>MADYKDDDDKSGRMATCWQALWAYRSYLIVFFVPILLLPLPILVPSKEAYCAYAIILMALFWCTEALPLAVTALFPLILFPMMGIVDASEVAVEYLKDSNLLFFGGLLVAIAVEHWNLHKRIALRVLLIVGVRPAPLILGFMLVTAFLSMWISNTATSAMMVPIAHAVLDQLHSSQASSNVEEGSNNPTFELQEPSPQKEVTKLDNGQALPVTSASSEGRAHLSQKHLHLTQCMSLCVCYSASIGGIATLTGTAPNLVLQGQINSLFPQNGNVVNFASWFSFAFPTMVILLLLAWLWLQILFLGFNFRKNFGIGEKMQEQQQAAYCVIQTEHRLLGPMTFAEKAISILFVILVLLWFTREPGFFLGWGNLAFPNAKGESMVSDGTVAIFIGIIMFIIPSKFPGLTQDPENPGKLKAPLGLLDWKTVNQKMPWNIVLLLGGGYALAKGSERSGLSEWLGNKLTPLQSVPAPAIAIILSLLVATFTECTSNVATTTIFLPILASMAQAICLHPLYVMLPCTLATSLAFMLPVATPPNAIVFSFGDLKVLDMARAGFLLNIIGVLVIALAINSWGIPLFSLHSFPSWAQSNTTAQCLPSLANTTTPSP[2x]

The solute carrier 13 (SLC13) family comprises electrogenic sodium ion–coupled anion cotransporters, segregating into sodium ion–sulfate cotransporters (NaSs) and sodium ion–di- and–tricarboxylate cotransporters (NaDCs). NaS1 and NaDC1 regulate sulfate homeostasis and oxidative metabolism, respectively. From an overall view, both the NaDC1 and NaS1 form a homodimer, and each protomer consists of 11 TMDs. The rest TMDs form the core domain that is responsible for substrate recognition and conformational change to complete the transport cycle.

In addition, we elucidated NaDC1’s outward-facing conformation, encompassing apo, citrate-bound, and N-(p-amylcinnamoyl) anthranilic acid (ACA) inhibitor–bound states. In this section, we will predominantly focus on the detailed structural analysis of the apo structure of NaDC1. Notably, the intracellular loop (residue 165 to 212 amino acids) of NaDC1 that connects the HPin and TM5 was poorly resolved because of its flexibility. In addition, the rest sequences of NaDC1 were clearly resolved, especially the preTM1 region (residue 1 to 12 amino acids) and intracellular loop 8 to 9 (IL8–9; residue 383 to 409 amino acids), of which the counterpart has not been resolved in human NaCT structure. The two hairpin segments (HPin and HPout), loop 5 (L5) between TM5a and TM5b, and L10 between TM10a and TM10b are essential for the coordination of substrate and sodium ions. Notably, the Ile550Val mutation occurred as a natural variant during the cloning of NaDC1 from a cDNA library, which was subsequently used to determine the protein’s structures. The polyalkylated tail of the lipid was firmly lodged within the hydrophobic pocket formed by HPin and TM4c, with additional stabilization facilitated through electrostatic interactions involving alkaline residues Arg112, His319, and Arg108. For illustrative purposes, we modeled a phosphatidic acid at this site; however, the precise phospholipid species necessitates further elucidation. In contrast to cholesterol binding to NaS1 C half (HPout and TM9c), phospholipid (modeled as phosphatidic acid) binds to the N half of NaDC1 (HPin and TM4c), which marginally propels the core domain toward the extracellular side. Although cholesteryl hemisuccinate, one of the cholesterol derivatives, was added during protein purification of NaDC1, the phospholipid site is still occupied by endogenous phospholipid-like molecule, indicating a higher affinity toward phospholipid molecules in this site of NaDC1.> MHHHHHHVSLDKAVIARLRKGGEEFEVLVDPYLARDLKEGKEVNFEDLLAAEEVFKDAKKGERASVDELRKIFGTDDVFEIARKIILEGEVQITAEQRREMLEAKRKQIINFISRNTIDPRTNAPHPPSRIERALEEAKVHIDIFKSVEAQVKDIVKALKPILPLKFEEMEIAIKIPPEHTGRAISALYNFGGVTREEWQRDGSWICVMRI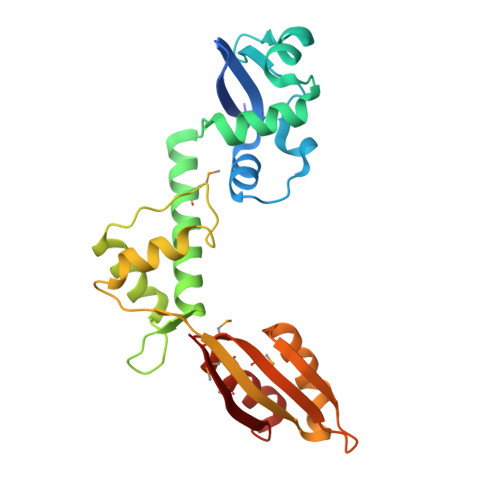PSGMYGDLMDLLGKVAKGEALTKVLRRIG>[2x]GMQGIAFQDAYPDDLSHCYGCGRNNEQGHQLKSY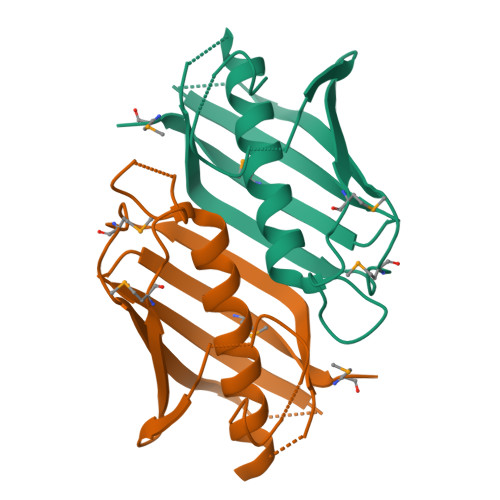WRGEQTIAHFMPKPFHTAIPGFVYGGLIASLIDCHGTGSASAAAQRALEQAGEQLDEPPRFVTAALNIDYLAPTPMGVELELVGEIKEVKPRKVVVEIALSADGKLCARGHMVAVKMPETMAATSA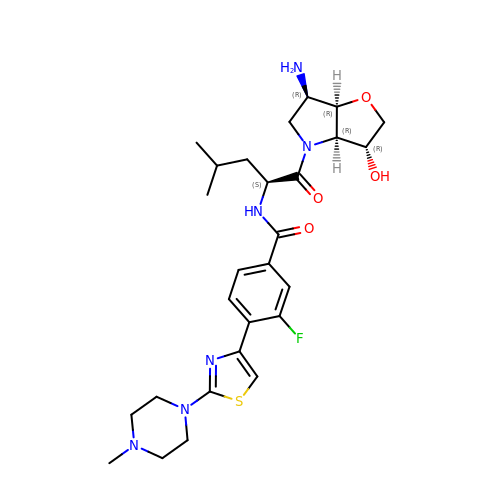~{N}-[(2~{S})-1-[(3~{R},3~{a}~{R},6~{R},6~{a}~{R})-6-azanyl-3-oxidanyl-2,3,3~{a},5,6,6~{a}-hexahydrofuro[3,2-b]pyrrol-4-yl]-4-methyl-1-oxidanylidene-pentan-2-yl]-3-fluoranyl-4-[2-(4-methylpiperazin-1-yl)-1,3-thiazol-4-yl]benzamide | C27 H37 F N6 O4 S | ZHJAUJFKEWMTLB-WPMOPGCQSA-N>[2x]MGSSHHHHHHSSGRENLYFQGEYDYTDFINYYDKFKVIVYNVLKKLPLNDEIRKPVIEYYLNCIDYNVKKGKHIRGKILVLISSLSSAYSNIKRDSIYLLGWVVEAIQALILIADDIMDSGKFRRGAPCWYI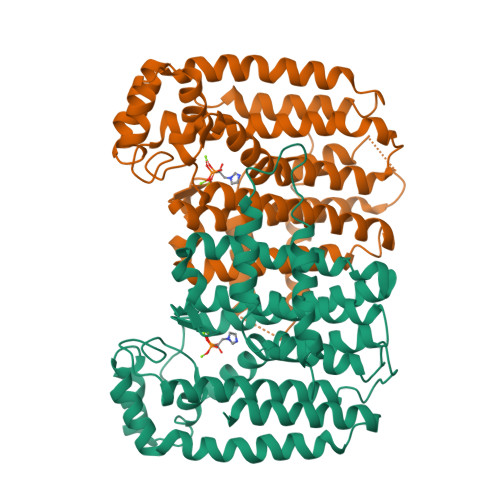VHGQSNAINDIFFLKMLSLSLIFELSSVFGNDIVMKIQKIYNESIFFTVLGQHLDLSYFDLSKADKISERYFSMVEMKTSRYTFYMPVFFGLTLSEIQVSSAQLNLIEAILYKLGEFYQVHNDVSDYLFNDSNADDICRFKLTWPLQKSFEIADEEMKLKISENYGKNSSLVKDCYNLLKINEHYLEYQRNALDYLIKLVKDITDDSLQKVFIHLIHQISELITNSRSNADSNNSL1-(quinoxalin-6-yl)methanamine | C9 H9 N3 | 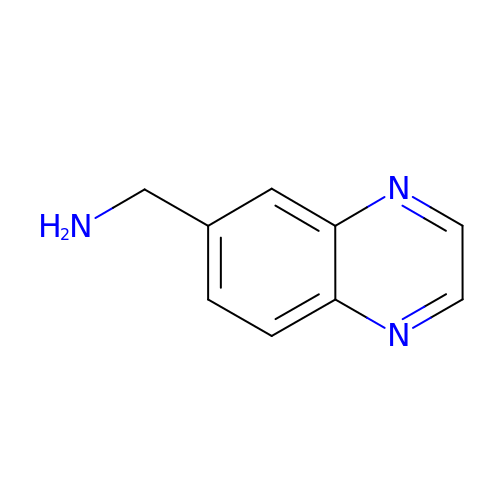LNYPHLYYOBNSPF-UHFFFAOYSA-N> SCSMPLGMQNKAISDSQITASSHLSNIFATWSPSQARLHLQGRTNAWRPRVSSAEEWLQVDLQKTVKVTGITTQGVKSLLSSMYVKEFLVSSSQDGRRWTLFLQDGHTKVFQGNQDSSTPVVNALDPPLFTRYLRIHPTSWAQHIALRLEVLG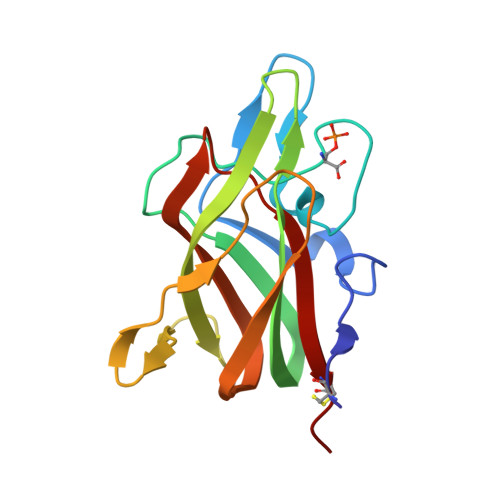CEAA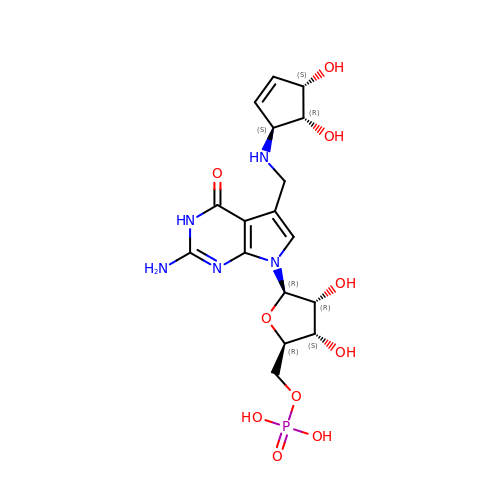2-amino-5-({[(1S,4S,5R)-4,5-dihydroxycyclopent-2-en-1-yl]amino}methyl)-7-(5-O-phosphono-beta-D-ribofuranosyl)-3,7-dihydro-4H-pyrrolo[2,3-d]pyrimidin-4-one | C17 H24 N5 O10 P | BSABGNSIPKXNDL-AEZJAUAXSA-N(2~{S})-2-acetamido-5-carbamimidamido-~{N}-prop-2-enyl-pentanamide | C11 H19 N5 O2 | 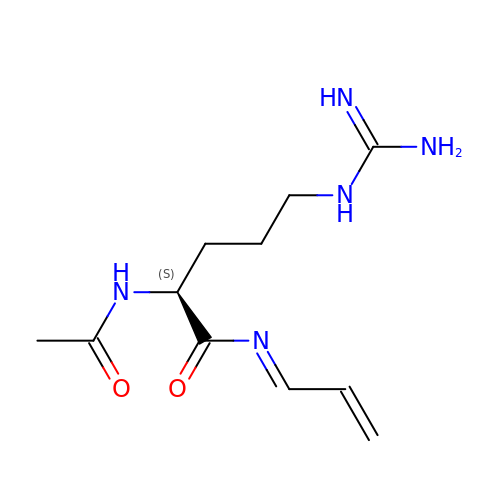SPVSLQNYRIRMJN-VYJZUSIPSA-N>[5x]MKADNPFDLLLPAAMAKVAEEAGVYKATKHPLKTFYLA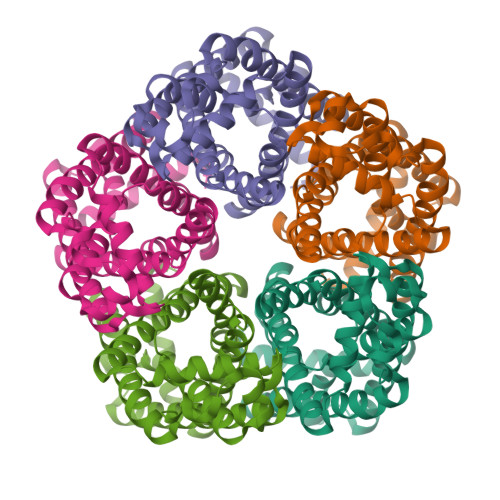ITAGVFISIAFVFYITATTGTGTMPFGMAKLVGGICFSLGLILCVVCGADLFTSTVLIVVAKASGRITWGQLAKNWLNVYFGNLVGALLFVLLMWLSGEYMTANGQWGLNVLQTADHKVHHTFIEAVCLGILANLMVCLAVWMSYSGRSLMDKAFIMVLPVAMFVASGFEHSIANMFMIPMGIVIRDFASPEFWTAVGSAPENFSHLTVMNFITDNLIPVTIGNIIGGGLLVGLTYWVIYLRENDHH> VTSYTLSDVVSLKDVVPEWVR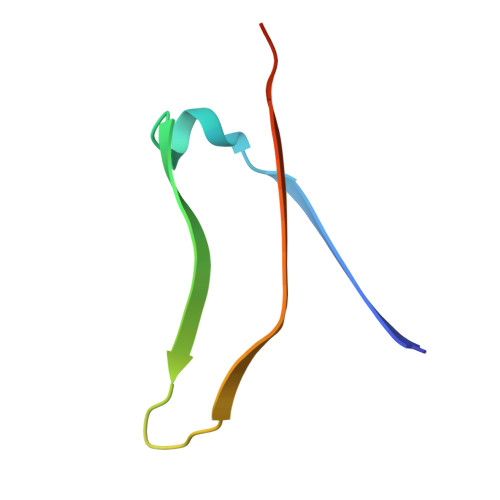IGFSATTGAEYAAHEVLSWSFHSELSGTSSS> AGSNGAQEKKYIVGFKQTMSTMSAAKKKDVIS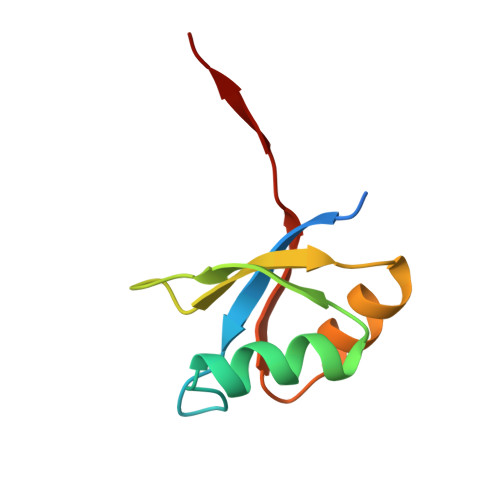EKGGKVQKQFKYVDAASATLNEKAVKELKKDPSVAYVEEDHVAHAY L and P function as the RNA polymerase complex, responsible for replicating and transcribing the viral genome. To catalyze the RNA synthesis in both replication and transcription, L sequentially consists of five domains: the RNA-dependent RNA polymerase domain (RdRp), polyribonucleotidyl transferase domain (PRNTase), connector domain (CD), methyltransferase domain (MTase), and C-terminal domain (CTD). P harbors an oligomerization domain (POD) for self-oligomerization, and the oligomeric P attaches to RdRp of L, tethering the polymerase to NC to extract the RNA strand for both replication and transcription. Here, we resolved two L–P complex conformations from the mumps virus (MuV), a typical member of nsNSVs, via cryogenic-electron microscopy.

In both conformations, parallel P tetramers are revealed around MuV L, which, together with structures of other nsNSVs, demonstrates the diverse origins of the L-binding X domain of P. Our study links varying structures of nsNSV polymerase complexes with genome replication and transcription and points to a sliding model for polymerase complexes to advance along the RNA templates. In cryo-EM maps, four P molecules assemble like a kettle spout stably anchored to L. Our cryo-EM structures capture the clear interface between two P molecules (depicted as P1 and P4, respectively) and L, involving the RdRp, POD, PLinker2, and PCTD regions. In this study, we observed that P tetramerizes more probably in a parallel pattern when constituted in complex with L. Due to the moderate resolution of P tetramer, we could not recognize the kink at Gly246, the unique feature to identify the helix orientation, and we could not rule out the possibility of MuV P tetramer in an anti-parallel configuration. The oligomerization forms of P in nsNSVs may depend on different conditions. Therefore, the involvement of L may guide the assembly of P monomers in EBOV, MuV, and others. Residues from 249 to 299 of P are the major region interacting with L.

>[4x]MDQFIKQDETGDLIETGMNVANHFLSTPIQGTNSLSKASILPGVAPVLIGNPEQKNIQHPTASHQGSKTKGRGSGVRSIIVSPSEAGNGGTQIPEPLFAQTGQGGIVTTVYQDPTIQPTGSYRSVELAKIGKERMINRFVEKPRTSTPVTEFKRGGPGAAAQGQTIQEEGIDGNGASAGSKERSGSLSGATLYAHLSLPQQDSTPANVGIAPQSAISANEIMDLLRGMDARLQHLEQKVDKVLAQGSMVTQIKNELSTVKTTLATIEGMMATVKIMDPGNPTGVPVDELRRSFSDHVTIVSGPGDVSFSSSEKPTLYLDELARPVSKPRPAKQTKSQPVKDLAGQKVMITKMITDCVANPQMKQAFEQRLAKASTEDALNDIKRDIIRSAI> MSRRVVRQSKFRHVFGQAAKADQAYEDIRVSKVTWDSSFCAVNPKFLAIIVEAGGGGAFIVLPLAKTGRVDKNYPLVTGHTAPVLDIDWCPHNDNVIASASDDTTIMVWQIPDYTPMRNITEPIITLEGHSKRVGILSWHPTARNVLLSAGGDNVIIIWNVGTGEVLLSLDDMHPDVIHSVCWNSNGSLLATTCKDKTLRIIDPRKGQVVAEQARPHEGARPLRAVFTADGKLLSTGFSRMSERQLALWDPNNFEEPVALQEMDTSNGVLLPFYDPDSSIVYLCGKGDSSIRYFEI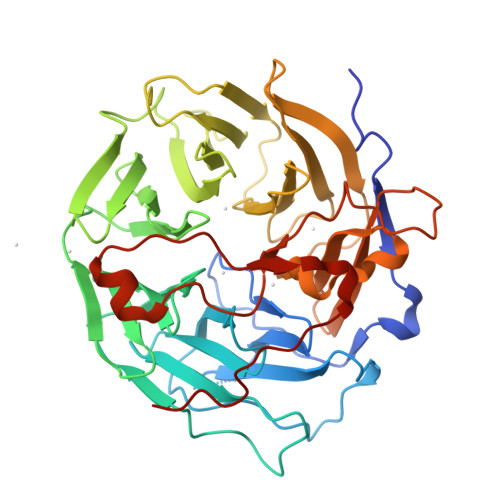TDEPPFVHYLNTFSSKEPQRGMGFMPKRGLDVSKCEIARFYKLHERKCEPIIMTVPRKSDLFQDDLYPDTPGPEPALEADEWLSGQDAEPVLISLRDGYVPPKHRELRVTKRN> MHHHHHHMPIIEQVRAREILDSRGNPTVEVEVALIDGTFARAAVPSGASTGEHEAVELRDGGDRYGGKGVQKAVQAVLDEIGPAVIGLNADDQRLVDQALVDLDGTPDKSRLGGNAILGVSLAVAKAAADSAELPLFRYVGGPNAHILPVPMMNILNGGAHADTAVDIQEFMVAPIGAPSFVEALRWGAEVYHALKSVLKKEGLSTGLGDAGGFAPDVAGTTAALDLISRAIESAGLRPGADVALALDAAATEFFTDGTGYVFEGTTRTADQMTEFYAGLLGAYPLVSIEDPLSEDDWDGWAALTASIGDRVQIVGDDIFVTNPERLEEGIERGVANALLVKVNQIGTLTETLDAVTLAHHGGYRTMISHRSGETEDTMIADLAVAIGSGQIKTGAPARSERVAKYNQLLRIEEALGDAARYAGDLAFPRFACETK

Enolase, a ubiquitous enzyme, catalyzes the reversible conversion of 2-phospho­glycerate (2PG) to phospho­enolpyruvate (PEP) in the glycolytic pathway of organisms of all three domains of life. Here we present structural snapshots of Mycobacterium tuberculosis (Mtb) enolase in apo, PEP-bound and two 2PG-bound forms as it catalyzes the conversion of PEP to 2PG. MtEno has a topology similar to other enolase structures, a smaller N-terminal domain and a larger C-terminal domain. The crystal and the cryoEM structures (enzyme in solution, frozen) along with the biochemical studies clearly demonstrate that the functional unit of MtEno is an octamer.

Tautomerization resonance is accelerated on acidification of the carboxyl group of 2PG which is accomplished through its lone-pair-mediated coordination with both the Mg2+ ions and the transfer of a proton from His154 onto the nearest oxygen linked to the phosphate moiety. To find out if the exact reverse of this reaction occurs during the conversion of PEP to 2PG, we systematically mutated each of the residues Ser42, Asp241, Glu163, Glu204 and Lys335 to alanine, compared their activity with wild type MtEno, and elucidated the structures of three of them [Figs. 4(a) and 4(b)]. Notably, the K335A mutation disrupts the nucleophilic (proton) substitution, the E204A mutation defuncts enolation capacity, D241A should make the MgA 2+ coordination in the active site highly improbable and S42A should absolve the MgB 2+ coordination.>MERPAILPSGQILSNIEVHSHRALFDIFKRFRSDDNNLYGAEFDALLGTYCSTLSLVRFLELGLSVACVCTKFPELSYVAEGTIQFEVQQPMIARDGPHPADQPVHNYMIKRLDRRSLNAAFSIAVEALGLISGENLDGTHISSAMRLRAIQQLARNVQAVLDSFERGTADQMLRVLMEKAPPLSLLAPFTLYEGRLADRVACAALVSELKRRVRDDTFFLTKHERNKDAVLDRLSDLVNCTAPSVAVARMTHADTQGRPVDGVLVTTAGVRQRLLHHVLTLADTHADVPVTYGEMVIANTNLVTALVMGKAVSNMDDVARYLLGGEPAPDDGKPVGSARVRADLVVVGDRLVFLEALEKRVYQATQVPYPLVGNLDVTFVMPLGVFKPAADRYARHAGSFAPTPGLPDPRTHPPRAVHFFNKDGVPCHVTFEHAMGTLCHPSFLDVDATLAALRQEPAEVQCAFGAYVADARPDALVGLMQRFLEEWPGMMPVRPRWAAPAAADQLLAPGNADLRLELHPAFDFFVAPEVDVPGPFAVPQVMGQVRAMPRIINGNIPLALCPVDFRDARGFELSVDRHRLAPATVAAVRGAFRDANYPMVFYIIEAVIHGSERTFCALARLVAQCIQSYWRNTHNAAFVNNFYMVMYINTYLGNGELPEDCAAVYKDLLEHVHALRRLIGEFTLPGDPLGNQPQEELNHALADATLLPPLIWDCDPILYRDGLAERLPELRVNGAHFQHILWVEMAQVNFRNVGGGLVHNRPVRNENQPLHPHHDAEWSVLSKIYYYAVVPAFSRGNCCTMGVRYDRVYQLVQTMVVPETDEEVGTDDPRHPLHPRNLVPNSLNVLFHNACVAVDADAMLILQETVTNMAERTTPLLASVAPDAGMATVATRDMRTHDGSLHHGLLMMAYQPNDATLLEGAFFYPAPVNALFACADHLGAMRDVGAEVRAAAQHVPCVPHFLGANYYATVRQPVAQHAAQSRADENTLSYALMAGYFKMSPVAFTHQLRRQLHPGFALTVVRQDRFATENVLFAEKASESYFMGQMQVARTESGGGLHLQLTQPRANVDLGVGFTAAYAAAALRAPVTDMGNLPQNLFATRGAPPMLDADADDYLRRTVNAGNRLAPVPVFGQMLPQVPAGLARGQQSVCEFIATPVSVDLAYFRRACNPRGRAAGEVHGEEGLMFDHSHADPAHPHRATANPWASQRHSYADRLYNGQYNMSGPAYSPCFKFFTPAEAVAKSRGLARLIADTGAAASPTSNGEYQFKRPVGAGELVEDPCALFQEAYPPLCASDSALLRTPLGAEEHFAQYLIRDESPLKGCFQHASA[16x];>[10x]MEVDIALPTLSPGDLSALQRCEGRVVFLETLRRHATLREVALPCGGDVLAAMAAYRRRFAAVITRVTPHRMLATPLGVGGRGQSLVLQNTGPFDLTNGDHVCLVPPLLGDECLRLTSANLELRFPMTLPLAQARELTARVVARAAETLRGGAPARGADVVFSNGRRYQLPPPHRDNAEAATRSLVLNMIFLLNEGAVILLSLIPNLLTLGAQDGYANAVIQLGSATRELGQLVRQPPPPLPQDHARRFCVFEALEAWIASASRLGDTLGTRPVARVCIFDGPPTVPPGEKAAVVEV;> MDAHIANETKQQMTRFAPALVHVIVPDPLLARAGVDPLAPFAAHAQTRYHGSGVCEPWVSVFAGHVQTGAVESVLTLPPLQRPRGPGGLFVSLPLALGAHFDGFTTAALRVGARELVFTYDELLPARTRYNVDGERLERLCRQFANYARARRVAPAVAAAGGHIDALLPPAAATIDGEAQLTRGGFDDPAAPHARDADREILSLVRRAAELVAARHPVRSHVASGLMQGALARRGGGGDGAGALEAAATVPAPAAREDANGGGAAWRDELLLTPQDPRPLTALDWLDAGYAALAGGDAPAHVWRRRPVSLVARRHYQTGETFVVVAYEHSTAWGGRRGPRGEPLARVLAEECERHGVEHPRALPAEARRELVRRHAELAVPLGDEEPPLPVFDATAELVLLERFRNACVRALLAGVRESVRREPRMRQIIEFAIRPRDREAVLDVAGRAPALLDAFARRLEHTPAREMVDSGLMTAAAAHLAARATAGYVTFESGPLLGGVFLFDYYSAGGEVIRVTRAPLAVAVEPATRGQFACRFRGASHRCLPGESYAYLCVGVSRDLRALVVLPGGFGFFATLRLEWPAALVDPVLERLCRRV;>[15x]MSFDPNNPRTITAQTLEGALPVDILLRLNRATGLQMDAAEAHAIVEDARRTLFIGTSLALVNLRRAHDKHLVERQPMFATSDYSSWARPTVGLKRTFCPRPPP;>[5x]MSVQIGNGLLMVVAPGTLTVGSARARLIRQVTLADFCEPQAERPGLVVLALRHPADLAGAAYAATPPGKNHRDLEEAWLALDEGGRGLGGDGIRASVVSLNFLVAAAENADDALRAHVTTNYRDRRTAARLERFATVLRAMIRSHVFPHRALHVLGGLLGHVTQDRLASVTCVARGDQEAARTNDMAARRSQVHVPACALMDVDRELRLGGDDGLRFAYLVFVYTQRHRREALRVHVAVSRLPELGDALSFLLAGTRVDNAIHGTDEADAPAAPAAAAAFPAYLFNDPRSARCPTGRLNTPAAEALPVWAPDMRGRATRNSCMYAAYVRLGTVERVVRRAERCGSVDLPLAHMERFTWDVGAWEECFF;>[2x]MDRAWFAFEAAAIPGSARHFIAPPFPVGFWARPGFGEGLDARLALAHANARRRAAAAALDNAMAAGARLEAEVDEQLRPLERQVERVAEALVVLEETARAAEEADAARAAEEAPEATAAADEGREVQIAKNDVALAYDANLSLDFLAMVYAARGAASGVLFGTWYATLQATLVAERPQVSRAIDSRDGRMSRTFMGVTTTALQACGRLYVGNRHYSALESAALCLHLVHRARQGPGAAGAAAPLGIADLLERVPEYLDALSQALAEGGRISYRYNYARVPREQLHGRYALEGHSVLAALARLRVVPGANVGANEVDGAGFVDEVNRAAAAFLGRGQNLFLGEDAPLLRATVNTITGLLLLRRLLHNGNVYGDRLRNNFQLGALVPNAPPPRGASGDAPASRSGDGNLRFLLAHYVVVAYRADERTELTQLFPGLAALALDAHSIRARVQRHQLNLVRLVALELQNRQRVTAPVNEVIAAHDAVAVQYEEGLGLLLQQPHLRNAADKRLGQFGVSSDYDLLYFLCLGYIPQFAAA;>RVVESDTLINRRYMRATGLGALALLIAACRLIARRLRETRTTLKGSARRFNVDLFQVRLILG[2x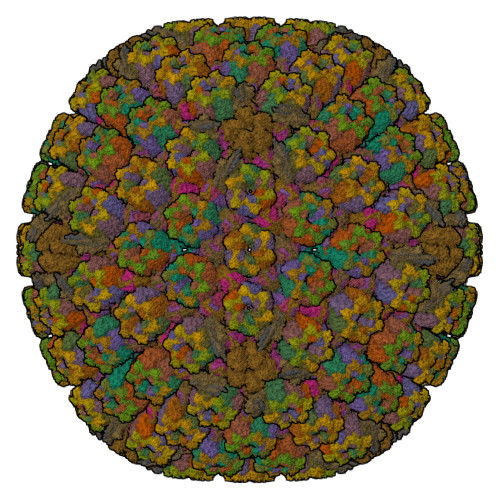]> GGLEKDFLPLYFGWFLTKKSSETLRKAGQVFLEELGNHKAFKKELRHFISGDEPKEKLELVSYFGKRPPGVLHCTTKFCDYGKAAGAEEYAQQEVVKRSYGKAFKLSISALFVTPKTAGAQVVLTDQELQLWPSDLDKPSASEGLPPGSRA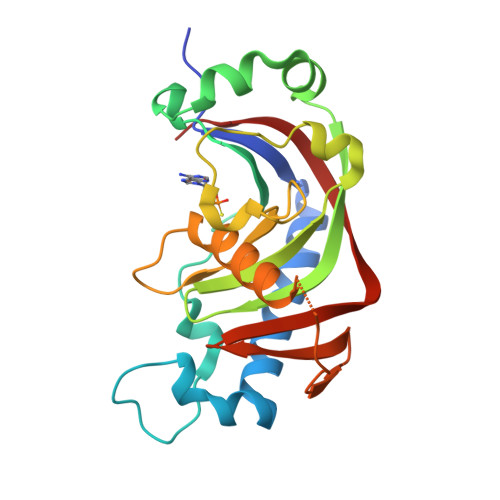SVTLGCAADVQPVQTGLDLLDILQQVKGGSQGEAVGELPRGKLYSLGKGRWMLSLTKKMEVKAIFTGYYG>SAAEASKKPRQKRTATKAYNVTQAFGRRGPEQTQGNFGDQELIRQGTDYKHWPQIAQFAPSASAFFGMSRIGMEVTPSGTWLTYTGAIKLDDKDPNFKDQVILLNKHIDAYKTFP[2x]

The SARS-CoV-2 nucleocapsid protein is a multifunctional protein with potential primary functions of binding to the viral RNA genome and packing it into a long helical nucleocapsid structure or RNP complex. The SARS-CoV-2 nucleocapsid protein consists of five domains: an N-terminal tail region (residues 1 to 40), an N-terminal RNA binding domain (residues 41 to 173, termed N-NTD), a Ser/Arg-rich linker region (residues 174 to 249, termed LKR), a C-terminal dimerization domain (residues 250 to 364, termed N-CTD), and a C-terminal intrinsically disordered region (residues 365 to 419, termed IDR). The N protein mediates ribonucleoprotein (RNP) complex formation via two key steps: packaging of the viral RNA genome and self-assembly of oligomerizations. Previous studies suggest that the coronavirus nucleocapsid contains multiple RNA binding sites, including the NTD, CTD, and C-terminal IDR regions.

To determine the precise structural information of the novel coronavirus SARS-CoV-2 N-CTD, we solved the N-CTD structure at a resolution of 2.0 Å with X-ray crystallography. One N-CTD monomer is composed of three 310-helices, five α-helices, and two β-strands, with an additional N-terminal α0-helix in the partial electron density of the traced molecule. Two N-CTD monomers utilize three regions to form a stable symmetrical dimer, with a buried surface area of 2618 Å2 (of the 8026 Å2 monomer surface) (calculated by the online PISA server). First, the most distinctive feature is the antiparallel four-stranded β-sheet that has domain swapping interactions between the two monomers. Second, residues F346, L353, V350, and I357 of the longest α5-helix form multiple intermolecular hydrophobic interactions with residues T329, M322, and I320 in the β1-strand. Last, the α1 helix forms a strong hydrophobic interaction with other monomer α4 helixes, like two clip-bars, to firmly fix the two monomers (i.e., A264-S312, Q260-S311, and Q260-Q306 interactions). SARS-CoV-2 N-CTDs form repeating cylindrical high-order structures with six dimers, which is slightly different from the SARS-CoV N-CTD octamer X-shaped high-order oligomer pattern. The dimer of SARS-CoV-2 N-CTD is shown as a cuboid shape containing an α-helix-rich side and a β-sheet side. The electrostatic surface suggests that the α-helix-rich side contains a positively charged channel, whereas the β-sheet side is a neutral surface. Nevertheless, the conserved positively charged channel of the α-helix-rich side is thought to be a potential RNA binding site in the SARS-CoV-2 N-CTD.> WVIVVGVIGVIG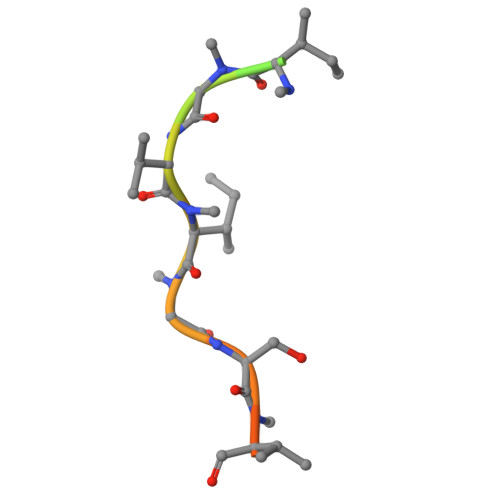SVMSTE> GPHMFEARLVQGSILKKVLEALKDLINEACWDISSSGVNLQSMDSSHVSLVQLTLRSEGFDTYRCDRNLAMGVNLTSMSKILKCAGNEDIITLRAEDNADTLALVFEAPNQEKVSDYEMKLMDLDVEQLGIPEQEYSCVVKMPSGEFARICRDLSHIGDAVV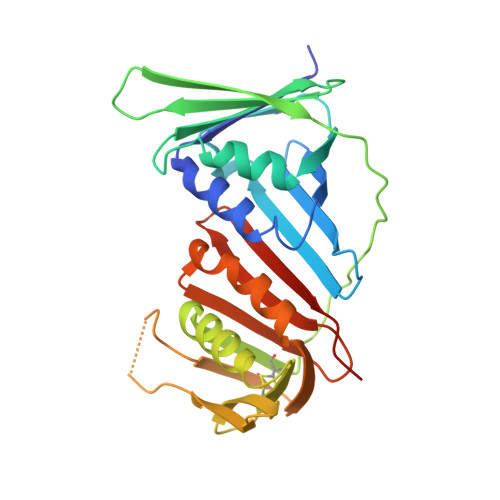ISCAKDGVKFSASGELGNGNIKLSQTSNVDKEEEAVTIEMNEPVQLTFALRYLNFFTKATPLSSTVTLSMSADVPLVVEYKIADMGHLKYYLAPKIEDEEGS>[2x]GSKGVSDLLGFKIFGMPLPLYAFALITLLLSHFYNALPTDIVGGFAIMFIIGAIFGEIGKRLPIFNKYIGGAPVMIFLVAAYFVYAGIFTQKEIDAISN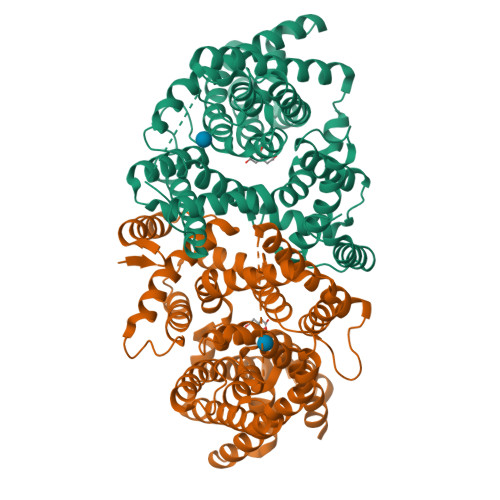VMDKSNFLNLFIAVLITGAILSVNRRLLLKSLLGYIPTILMGIVGASIFGIAIGLVFGIPVDRIMMLYVLPIMGGGNGAGAVPLSEIYHSVTGRSREEYYSTAIAILTIANIFAIVFAAVLDIIGKKHTWLSGEGELVRKASFKVEEDEKTGQITHRETAVGLVLSTTCFLLAYVVAKKILPSIGGVAIHYFAWMVLIVAALNASGLCSPEIKAGAKRLSDFFSKQLLWVLMVGVGVCYTDLQEIINAITFANVVIAAIIVIGAVLGAAIGGWLMGFFPIESAITAGLCMANRGGSGDLEVLSACNRMNLISYAQISSRLGGGIVLVIASIVFGMMIPR> MKKLIPILEKIPEVELPVKEITFKEKLKWTGIVLVLYFIMGCIDVYTAGAQIPAIFEFWGRIGTLITLGIGPIVTAGIIMQLLVGSGIIQMDLSIPENRALFQGCQKLLSIIMCFVEAVLFVGAGAFGILTPLLAFLVIIQIAFGSIILIYLDEIVSKYGIGSGIGLFIAAGVSQTIFVGALGPEGYLWKFLNSLIQGVPNIEYIAPIIGTIIVFLMVVYAECMRVEIPLAHGRIKGAVGKYPIKFVYVSNIPVILAAALFANIQLWGLALYRMGIPILGHYEGGRAVDGIAYYLSTPYGLSSVISDPIHAIVYMIAMIITCVMFGIFWVETTGLDPKSMAKRIGSLGMAIKGFRKSEKAIEHRLKRYIPPLTVMSSAFVGFLATIANFIGALGGGTGVLLTVSIVYRMYEQLLREKVSELHPAIAKLLNK;> MKTDFNQKIEQLKEFIEECRRVWLVLKKPTKDEYLAVAKVTALGISLLGIIGYIIHVPATYIKGILKPPTTPRV;> MSK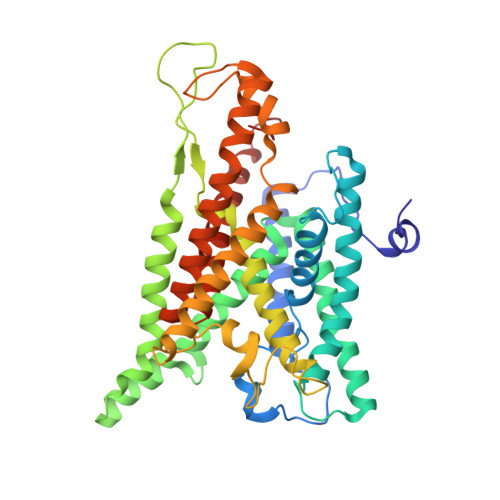REETGLATSAGLIRYMDETFSKIRVKPEHVIGVTVAFVIIEAILTYGRFL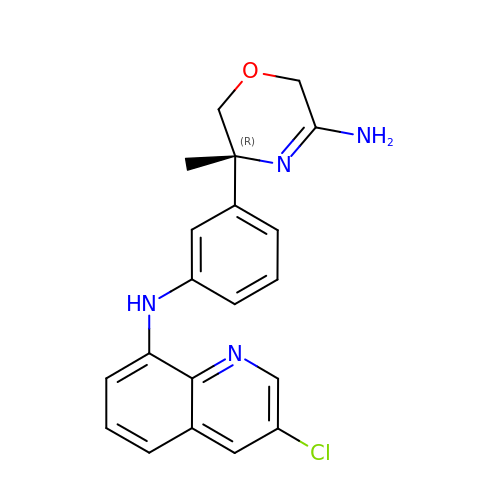(5~{R})-5-[3-[(3-chloranylquinolin-8-yl)amino]phenyl]-5-methyl-2,6-dihydro-1,4-oxazin-3-amine | C20 H19 Cl N4 O | MISZEAYFRRVHET-FQEVSTJZSA-N> GPGSLSQASADLEATLRHKLTVMYSQINGASRALDDVRNRQQDVRMTANRKVEQLQQEYTEMKALLDASETTSTRKIKEEEKRVNSKFDTIYQILLKKKSEIQTLKEEIEQSLTKRDEFEFLEKASKLRGISTKPVYIPEVELNHKLIKGIHQSTIDLKNELKQCIGRLQELTPSSGDPGEHDPA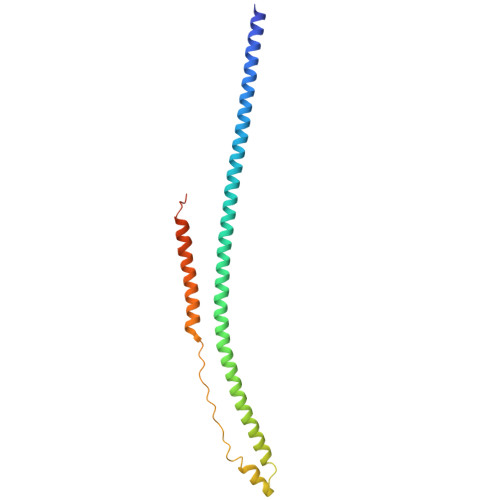STHKSTRP3-(1H-pyrazol-4-yl)benzoic acid | 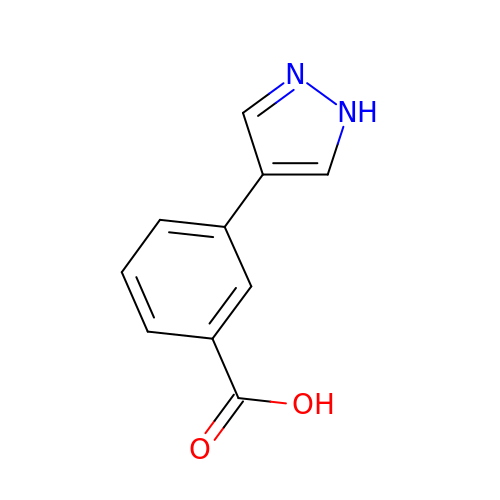C10 H8 N2 O2 | BXSUQWZHUHROLP-UHFFFAOYSA-N> MSLDVTALLERGRTLATPVLRAAVDRLAPPMDTVAAYHFGWIDAQGNPADGDGGKAVRPAL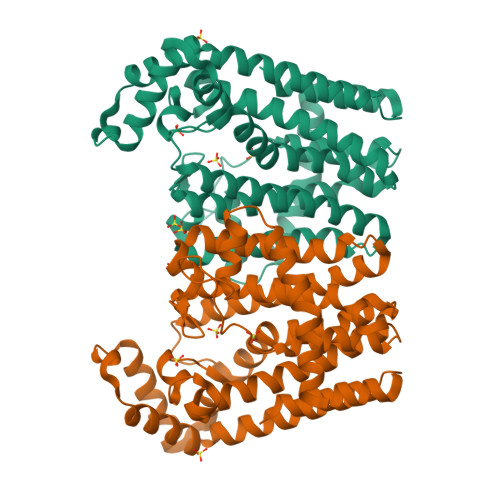AVLSAEVTGAAPEVGVPGAVAVELVHNFSLLHDDLMDGDEQRRHRDTVWKVHGPAQAILVGDALFALANEVLLELGTVEAGRATRRLTKASRSLIDGQAQDISYEHRDRVSVEECLEMEGNKTGALLACASSIGAVLGGADERTADTLEKYGYHLGLAFQAVDDLLGIWGDPDATGKQTWSDLRQRKKSLPVVAALAAGGAASERLGEILTADAKASDFANFSEEEFAARAALIEEAGGREWTADEARRQHTIAIEALDAVDMPDRVRDRFTALADFVVVRKREGHHHHHH>MGKIVEIHPTTRHEGHTKLVLKVDDEGIVEKGAYLSVTPVRGFEKFLVGKPAEFAPIAVSRFCGICPVAHATSAVEAIEDACDITPPKDGLLLRELCGIGNKMHSHPLHQFLISPDYVPKDDSNEFIKRVQAMRRIGQYIVDAVGGEAIHSPNIKVGGMAKQITESTKAKMYYKCKEYEKLAKEQLEYLIPIFESRTLNDGTELPEKLGYHDFGYIATHPTYGDRTKIDQDKVVEYTPFDVYDKDVAIQSSTTVPTYNGRLMEVGPRARFSKFFDFKEKGAMALHIARAYEISVLVKRAMEILDELNVNGKTMSDEPIVGDGEKLGLGVHEAARGHNTHQAVIDKDGNIVYYNAIVATTWNIPVISKAVEGTHYKFAEHIVRAYDPCISCATHMIIKDYDDKIIGEKILK[4x];>MDPFGKYKTVVSARAADKTILKKCQDGGIVSAAYIYGLENGLLDGVIVADKDDKLQTTPKVATTVDEVLEAAGTKYTVCPTISVIKSAVREYGCEKLGVVGTPCQIIATRKLMKYPIGFRHVPDKLALIVGIFCMENFPYNGMKTIIEEHCGIKMEDVAKTDIGKGKFWVYSKWGDVKSIKLKETHPYEQQSCHVCMDYTAELADISTGSVGSPDGWSTVFIRTAQGEEFFNKMVEAGALEVKPIEEVKPGLGLVEKLSLTKKEKNAKEIEHRKEIGLPVPY[4x];>[4x]MVKIAHIHLCGCTGCLISLADTYEQLLDILNSVELVYALTLVDEKTEIRETDDKILIEREIPDDIDIALVEGSVCLEDEHSMKDVFDARRKSKIVVALGACAATGGITRFCRGGQMSKPVHSSFVPIGDLIKVDLALPGCPPSPEALVNLITAALNGDTEYLEIYAELAKKTEACGCDLLVNVINKSLCMGCGSCAASCPTRAIEMIDGKPNVLKELCIKCGACSLQCPRIRFPKLIEEIE

FRHs catalyze the reversible H2 oxidation coupled to the reduction of coenzyme F420 (8‐hydroxy‐5‐deazaflavin, ΔG°′ = −10 kJ mol−1). The overall reaction requires three components: the large subunit (FRHA) that harbors the [NiFe] center and oxidizes H2, and the small subunit (FRHG), which contains three [4Fe–4S] clusters to transfer electrons to the flavin adenine dinucleotide (FAD) located in the F420‐reducing module (FRHB, harboring an additional [4Fe–4S] cluster). FRHABG dimerizes and forms dodecameric assemblies of about 16 nm in diameter with a spherical shape and a hollow core. Here, by characterizing the native hydrogenase from the marine methanogen Methanothermococcus thermolithotrophicus (belonging to the Methanococcales order), we provided an unprecedented functional understanding of this enzyme via a synergistic approach of biochemistry, X‐ray crystallography, and spectroscopy.

Despite its sequence conservation with the two other structural homologs, we found that the [NiFe]‐containing FRH from M. thermolithotrophicus (MtFRH) exhibits a dynamic equilibrium between a dodecameric and dimeric state in solution, as highlighted by size exclusion chromatography and native polyacrylamide gel electrophoresis (PAGE). It was therefore not surprising to observe several crystalline forms containing either a dodecameric cubic organization (MtFRHcube) or only a single FRH dimer (MtFRHdimer1 −3). Based on the four X‐ray crystallographic structures obtained, we confirmed that MtFRH shares the basic organization previously observed with an elementary dimer of FRHABG heterotrimers that further builds into a dodecameric unit. The electronic path is highly similar to structural homologs, despite variations in the occupancy of the protomer‐bridging [2Fe–2S] cluster and FAD, which is likely an artifact of purification or oxidative damage, as the only reducing agent used during purification and crystallisation was dithiothreitol. FRH structures are superimposable without any movements between functional domains. The only noticeable difference is an N‐terminal extension in FRHG that forms a β‐hairpin, interacting with a β‐sheet of FRHA, which may enhance the thermal stability of the enzyme.> SFAKGTNVLMADGSIECIENIEVGNKVMGKDGRPREVIKLPRGRETMYSVVQKSQHRAHKSDSSREVPELLKFTCNATNELVVRTPRSVRRLSRTIKGVEYFEVITFEMGQKKAPDGRIVELVKEVSKSYPISEGPERANELVESYRKASNKAYFEWTIEARDLSLLGSHVRKATYQTYAPILYENDHFFDYMQKSKFHLTIEGPKVLAYLLGLWIGDGLSDRATFSVDSRDTSLMERVTEYAEKLNLCAEYKDRKEPQVAKTVNLYSKVVRGNGIRNNLNTENPLWDAIVGLGFLKDGVKNIPSFLSTDNIGTRETFLAGLIDSDGYVTDEHGIKATIKTIHTSVRDGLVSLARSLGLVVSVNAEPAKVDMNGTKHKISYAIYMSGGDVLLNVLSKCAGSKKFRPAPAAAFARECRGFYFELQELKEDDY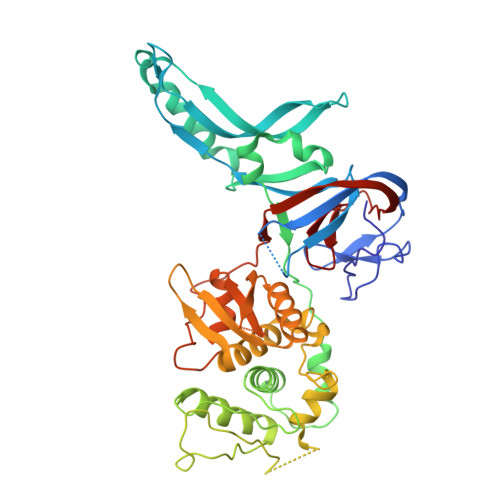YGITLSDDSDHQFLLANQVVVHN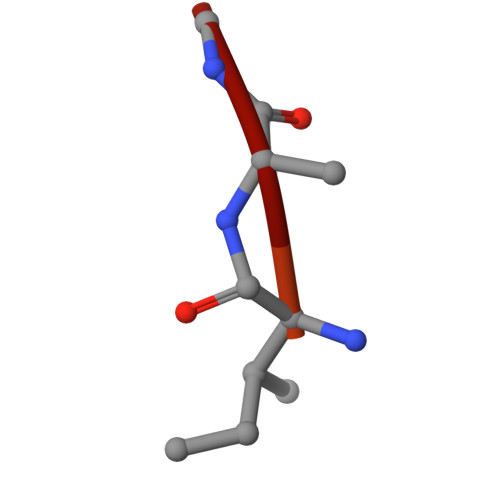> YPFVEPIRF>GHMGKVTKNSSSIKVVKLLVRLSDSVGYLFWDSATTGYATCFVFKGLFILTCRHVIDSIVGDGIEPSKWATIIGQCVRVTFGYEELKDKETNYFFVEPWFEIHNEELDYAVLKLKENGQQVPMELYNGITPVPLSGLIHIIGHPYGEKKQIDACAVIPQGQRAKKCQERVQSKKAESPEYVHMYTQRSFQKIVHNPDVITYDTEFFFGAAGSPVFDSKGSLVAMHAAGFAYTYQNETRSIIEFGSTMESILLDIKQRHKPWYEEVFVNQQDVEMMSDEDL[4x]

FAM111A (FAM111 trypsin-like peptidase A) is a serine protease involved in multiple cellular processes including antiviral defense and DNA replication. FAM111A contains a serine protease domain (SPD) with a conserved catalytic triad (His385, Asp439, and Ser541). The FAM111A SPD belongs to the S1 family of serine peptidases, which includes chymotrypsin, in the MEROPS database. Here, we show that FAM111A is a dimerization-dependent protease containing a narrow, recessed active site that cleaves substrates with a chymotrypsin-like specificity.

To mitigate the potential problem with protein production due to autocleavage, we generated the mutant SPD (S541A), which lacks the serine nucleophile of the catalytic triad, and performed crystallization trials with the purified protein. Our crystal structure of the SPD has revealed that it is a dimer with a coiled coil interface between the N-terminal α-helices within the SPDs. Overall, the individual SPD chains are similar to each other, with root mean square derivations (RMSDs) ranging from 0.15 Å to 0.3 Å over Cα atoms. Thus, we focused our analysis on chain D, which is the most complete, but our analysis is broadly applicable to all chains. Interestingly, a protrusion of β-strands (β2 and β10) buttressed by helices α2 and α5 yields a protease domain with an active site located at the bottom of a trench, whereas the active site of chymotrypsin is shallow and accessible for substrate engagement. This suggests that the FAM111A SPD active site architecture is tailored to cleave smaller substrates, such as linker regions or disordered substrates, and not globular proteins. FAM111A possesses an oxyanion hole formed by the backbone amide nitrogen of Ser541 and Gly539, as well as a P1 residue binding pocket (designated as the S1 pocket) similar to that of chymotrypsin. While the S1 pocket in FAM111A is about 0.5 Å narrower than that observed in chymotrypsin, it can still easily accommodate phenylalanine by allowing rotation of the peptide bond between Phe537 and Phe538. The loop L4, which is disordered in the monomeric SPD, is structured in the dimeric SPD and forms salt bridges with Lys348 and Lys345 of the dimerization partner through Glu415 and Glu416. Furthermore, the loop L4 contains Tyr414, which is positioned in the dimer structure adjacent to the loop L6 that is also unstructured in the monomeric SPD but structured in the dimeric SPD.>[6x]NYCNQMMKSRNLTKDRCKPVNTFVHESLADVQ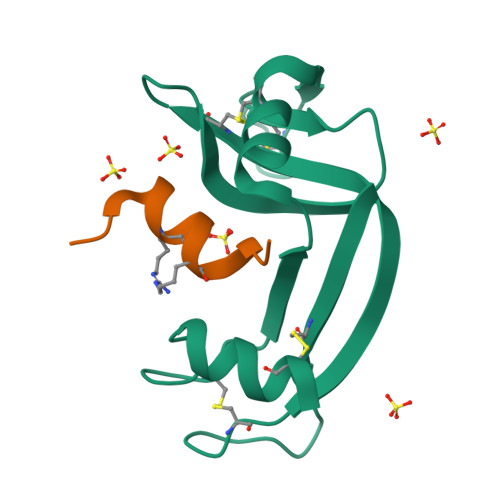AVCSQKNVACKNGQTNCYQSYSTMSITDCRETGSSKYPNCAYKTTQANKHIIVACEGNPYVPVHFDASV;>[6x]XKETAAALFERQHMDSX> GPLGSMASSNMKDETYYIALNMIQNYIIEYNTNKPRKSFVIDSISYDVLKAACKSVIKTNYNEFDIIISRNIDFNVIVTQVLEDKI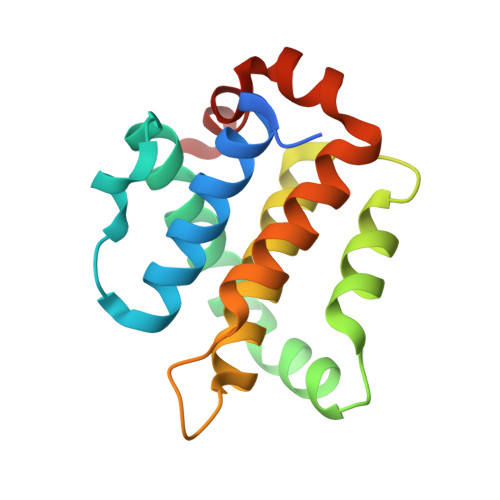NWGRIITIIAFCAYYSKKVKQDTSPQYYDGIISEAITDAILSKYRSWFIDQDYWNGIRIYKN>[2x]MRGSHHHHHHGSMSETAKKVIVGMSGGVDSSVSAWLLQQQGYQVEGLFMKNWEEDDGEEYCTAAADLADAQAVCDKLGIELHTVNFAAEYWDNVFELFLAEYKAGRTPNPDILCNKEIKFKAFLEFAAEDLGADYIATGHYVR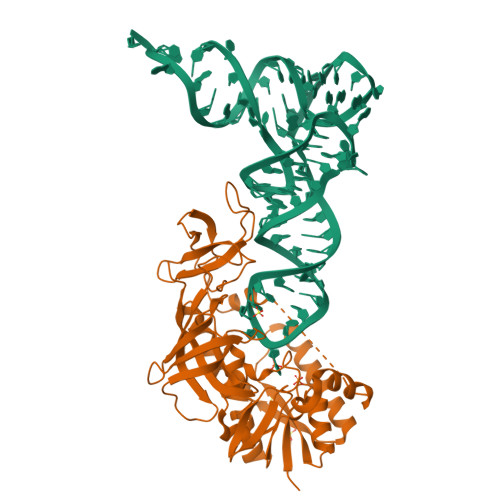RADVDGKSRLLRGLDSNKDQSYFLYTLSHEQIAQSLFPVGELEKPQVRKIAEDLGLVTAKKKDSTGICFIGERKFREFLGRYLPAQPGKIITVDGDEIGEHQGLMYHTLGQRKGLGIGGTKEGTEEPWYVVDKDVENNILVVAQGHEHPRLMSVGLIAQQLHWVDREPFTGTMRCTVKTRYRQTDIPCTVKALDDDRIEVIFDEPVAAVTPGQSAVFYNGEVCLGGGIIEQRLPLPV>[2x]AKPDRSSFVPSLFSKKKKNVTMRSIKTTRDRVPTYQYNMNFEKLGKCIIINNKNFDKVTGMGVRNGTDKDAEALFKCFRSLGFDVIVYNDCSCAKMQDLLKKASEEDHTNAACFACILLSHGEENVIYGKDGVTPIKDLTAHFRGDRCKTLLEKPKLFFIQACRGTELDDGIQ;>[2x]ANPRYKIPVEADFLFAYSTVPGYYSWRSPGRGSWFVQALCSILEEHGKDLEIMQ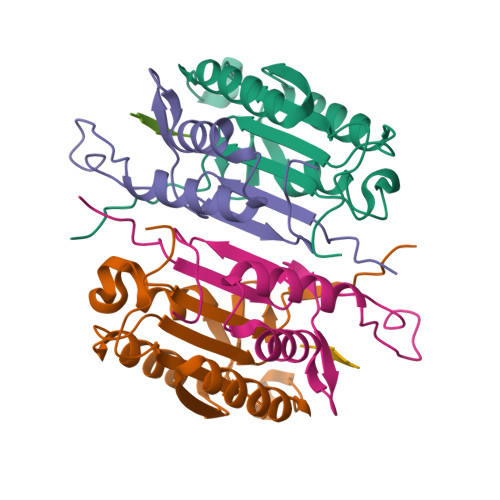ILTRVNDRVARHFESQSDDPHFHEKKQIPCVVSMLTKELYFSQ;>[2x]XYVAD> MYRNLYDTDNIIYSPEGRLYQVEYASEAIKQGTCAVAIKSKDYVVVSGLKKCISKLSFPQEKIFKIDDYIGISMSGITSDAKVLTKFMQNECLSHKFLYNENINIESLVRSVADKYQKNTQKSSKRAFGVGLMIAAYHNEPCIFETRPNGSYFEYDALSFGARSHASKTYLEKNLHLFEECSLEELILHCLKALKCSLSSESELTISNTALAVVGK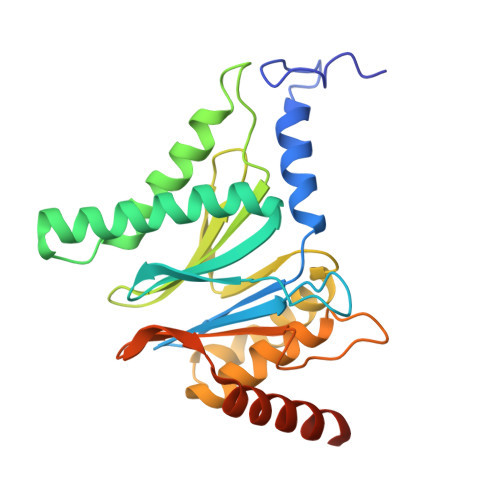NHPWQEISSLQLEEYLSKVKMDAEQEQVEENVQNEAN> TLPWDL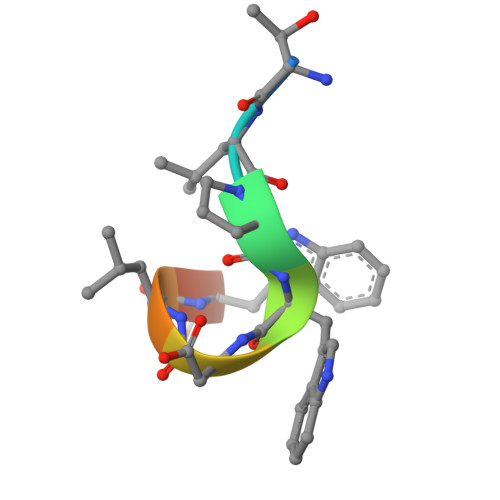WTT> 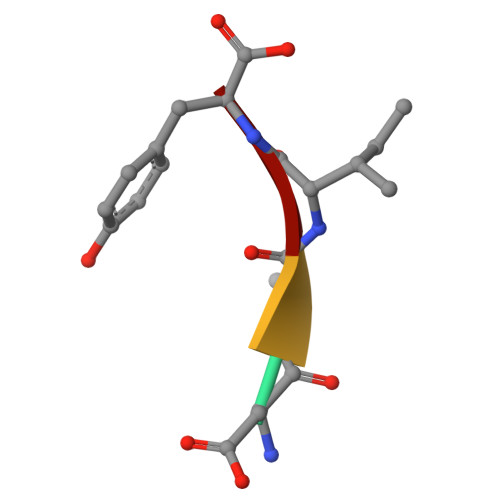DAIY> QSLRSSLLGLRQLLRELPGDEAPLDALAETVLALLAQYGSLRIAGLYRVRYDRTPEPQPLATLGEMPALDADDLLVRTCLERGELVSVRQELLERGEQRAHSAAAVCVPLVDTDGRILALLAVEQMPFFVFNERTFSLLAILAGHIADLLQSDRRALQLADIDAQRFSQYLKRSLLDARDHGLPACLYAFELTDARYGEEVQ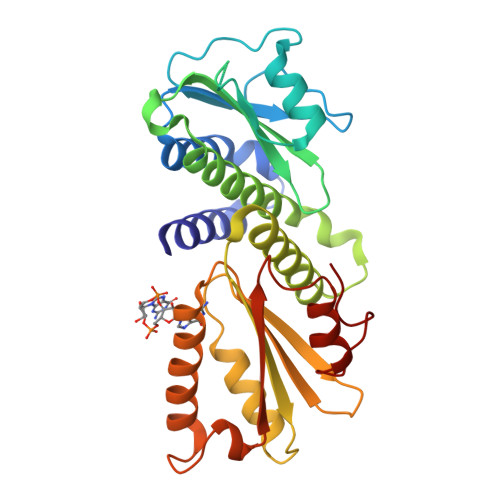RLLEGSQRGLDVQLRLRNDEGRRVLLVLLPLTSAEGSQGYLQRLRILFAERFGQARELESLGVRIRQYELDAGNDRQALGHFLFNECGLNDQQVAI> MMSREALQETLSAVMDNEADELELRRVLAACGEDAELRSTWSRYQLARSVMHREPTLPKLDIAAAVSAALADEAAPPKAEK;> MLTQEQDQQLVERVQRGDKRAFDLLVLKYQHKILGLIVRFVHDAQEAQDVAQEAFIKAYRALGNFRGDSAFYTWLYRIAINTAKNHLVARGRRPPDSDVTAEDAEFFEGDHALKDIESPER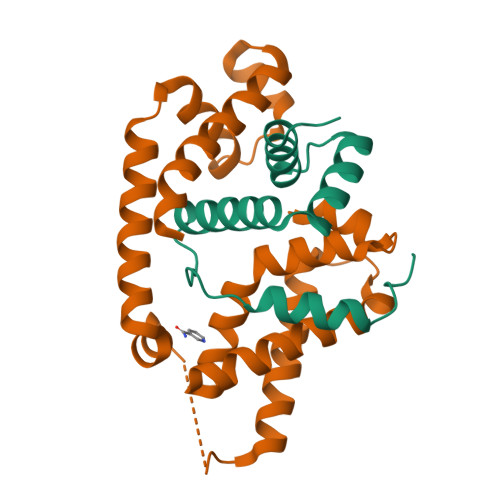AMLRDEIEATVHQTIQQLPEDLRTALTLREFEGLSYEDIATVMQCPVGTVRSRIFRAREAIDKALQPLLREA> MSTSTSQIAVEYPIPVYRFIVSVGDEKIPFNSVSGLDISYDTIEYRDGVGNWFKMPGQSQSTNITLRKGVFPGKTELFDWINSIQLNQVEKKDITISLTNDAGTELLMTWNVSNAFPTSLTSPSFDATSNDIAVQEITLMADRVI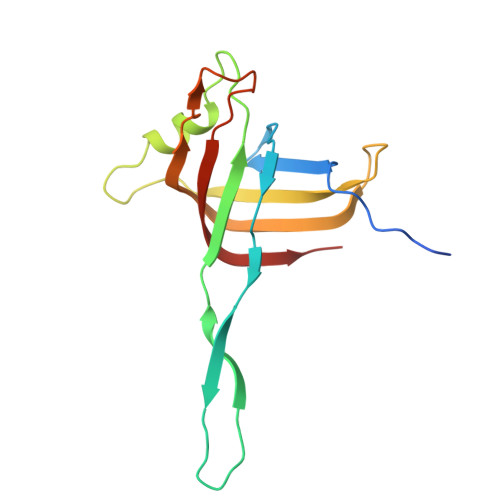MQAV> PAAAPGKNFDLSHWKLQLPDANTTEISSANLGLGYTSQYFYTDTDGAMTFWAPTTGGTTACSSYPRSELREMLDPSNSKVNWGWQGTHTMKLSGKTVQLPSSGKIIVAQI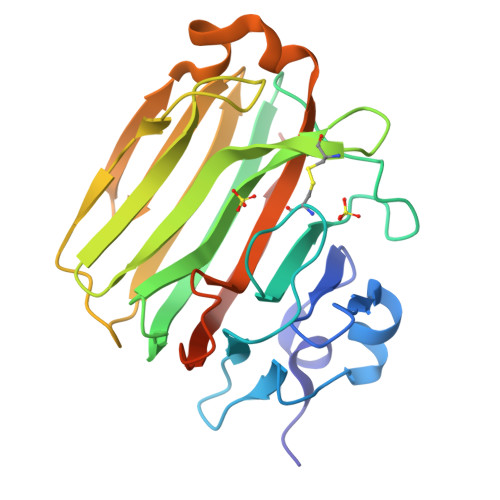HGIMDDGTCAPPLVKAVFQDGQLDMQVKQNSDGTGSDVHNYFTGIKLGDLYNMEIRVTDGVAYVTMNGDTRSVDFVGKDAGWKNLKYYFKAGNYVQDNTSTGGSAIAKLYSLSVSHSNLEHHHHHH>MGHHHHHHMMKFINIGYGNMVSAARIITIVSPDSAPIKRIIQDAREKGKLVDATHGRATAAVIITDSDHVILSSVQPETVANRLYG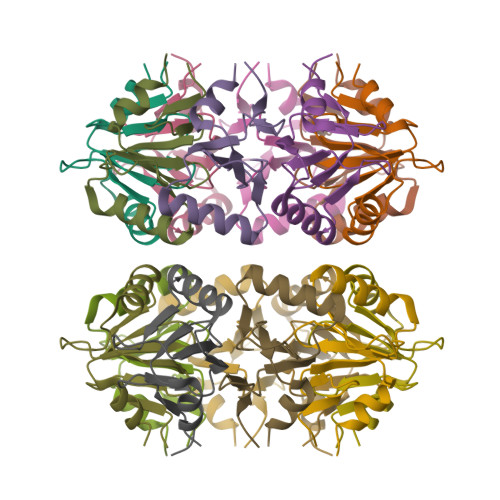SDDFSEEG[2x]TEM-1 β-lactamase degrades β-lactam antibiotics with a strong preference for penicillins. Sequence reconstruction studies indicate that it evolved from ancestral enzymes that degraded a variety of β-lactam antibiotics with moderate efficiency. This generalist to specialist conversion involved more than 100 mutational changes, but conserved fold and catalytic residues, suggesting a role for dynamics in enzyme evolution. The resurrected Precambrian β-lactamases were found to degrade both penicillin and third-generation antibiotics (such as CTX) with moderate catalytic efficiency.

By deliberately weighting and altering the conformational dynamics of a putative Precambrian β-lactamase, we engineer enzyme specificity that mimics the modern TEM-1 β-lactamase with only 21 amino acid replacements. In an effort to further validate the hinge-shift mechanism, we have engineered the minimum number of necessary substitutions in the ancestral GNCA β-lactamase, such that the designed mutant is closer, in its activity, to that of the specialist extant TEM-1 β-lactamase. We propose a detailed mechanism, according to which selected substitution mutations are applied to GNCA, which gradually drives its dynamics (DFI profile) towards that of TEM-1 β-lactamase. Indeed, we observed that mutations in sets X and Y, when combined together, bring the dynamics of GNCA closer to TEM-1 β- lactamase. Adding substitutions in set Z with the previous substitutions (set XYZ), we managed to shift the DFI profile of the engineered mutant towards that of TEM-1 β-lactamase beyond what was accomplished by the XY substitutions alone. The comparison of the flexibility profiles of the GNCA mutant with mutations from set XY and set Z together and the wild-type GNCA and TEM-1 β-lactamases show that the mutant successfully recapitulates the dynamics of TEM-1 β-lactamase. We observe that, as expected, the mutant GNCA-XYZ lies very close to the wild-type TEM-1 β-lactamase, which is an improvement over mutants with mutations from sets X and XY, suggesting that the ancestral variant GNCA-XYZ with merely 21 substitutions should degrade only penicillin with better efficiency than GNCA β-lactamase, mimicking the catalytic activity of TEM-1 β-lactamase. Therefore, using these 21 substitutions, we are able to dynamically replicate the effect of a total of 119 substitutions observed between GNCA and TEM-1 β-lactamase.

>[2x]MAAQLSEQLAELEKRSGGRVGVIVLDTATGRRIAYRGDERFPMMSTFKALLAAAVLARVDAGKERLGRRITYSKEDLVDYSPVTEKHVGDGMTVAELCEAAITLSDNTAANLLLEALGGPAALTAFLRSIGDEVTRLDRWEPELNEAAPGDERDTTMPAAMAATLRTLLLGDALSPASRQQLVDWLVANKTGGKLLRAGLPADWRIGDKSGAGEHGSRNIIAVIGPPGRAPIIVVIYLTESQVDADARDAVIAEVGRLVVEAFHHHHHH>[5x]MNESVKEIPDVLKSQCGFNCLTDISHSSFNEFRQQVSEHLSWSETHDLYHDAQQAQKDNRLYEARILKRANPQLQNAVHLAILAPNAELIGYNNQFSGRASQYVAPGTVSSMFSPAAYLTELYREARNLHASDSVYYLDTRRPDLKSMALSQQNMDIELSTLSLSNELLLESIKTESKLENYTKVMEMLSTFRPSGATPYHDAYENVREVIQLQDPGLEQLNASPAIAGLMHQASLLGINASISPELFNILTEEITEGNAEELYKKNFGNIEPASLAMPEYLKRYYNLSDEELSQFIGKASNFGQQEYSNNQLITPVVNSSDGTVKVYRITREYTTNAYQMDVELFPFGGENYRLDYKFKNFYNASYLSIKLNDKRELVRTEGAPQVNIEYSANITLNTADISQPFEIGLTRVLPSGSWAYAAAKFTVEEYNQYSFLLKLNKAIRLSRATELSPTILEGIVRSVNLQLDINTDVLGKVFLTKYYMQRYAIHAETALILCNAPISQRSYDNQPSQFDRLFNTPLLNGQYFSTGDEEIDLNSGSTGDWRKTILKRAFNIDDVSLFRLLKITDHDNKDGKIKNNLKNLSNLYIGKLLADIHQLTIDELDLLLIAVGEGKTNLSAISDKQLATLIRKLNTITSWLHTQKWSVFQLFIMTSTSYNKTLTPEIKNLLDTVYHGLQGFDKDKADLLHVMAPYIAATLQLSSENVAHSVLLWADKLQPGDGAMTAEKFWDWLNTKYTPGSSEAVETQEHIVQYCQALAQLEMVYHSTGINENAFRLFVTKPEMFGAATGAAPAHDALSLIMLTRFADWVNALGEKASSVLAAFEANSLTAEQLADAMNLDANLLLQASIQAQNHQHLPPVTPENAFSCWTSINTILQWVNVAQQLNVAPQGVSALVGLDYIESMKETPTYAQWENAAGVLTAGLNSQQANTLHAFLDESRSAALSTYYIRQVAKAAAAIKSRDDLYQYLLIDNQVSAAIKTTRIAEAIASIQLYVNRALENVEENANSGVISRQFFIDWDKYNKRYSTWAGVSQLVYYPENYIDPTMRIGQTKMMDALLQSVSQSQLNADTVEDAFMSYLTSFEQVANLKVISAYHDNINNDQGLTYFIGLSETDAGEYYWRSVDHSKFNDGKFAANAWSEWHKIDCPINPYKSTIRPVIYKSRLYLLWLEQKEITKQTGNSKDGYQTETDYRYELKLAHIRYDGTWNTPITFDVNKKISELKLEKNRAPGLYCAGYQGEDTLLVMFYNQQDTLDSYKNASMQGLYIFADMASKDMTPEQSNVYRDNSYQQFDTNNVRRVNNRYAEDYEIPSSVSSRKDYGWGDYYLSMVYNGDIPTINYKAASSDLKIYISPKLRIIHNGYEGQKRNQCNLMNKYGKLGDKFIVYTSLGVNPNNSSNKLMFYPVYQYSGNTSGLNQGRLLFHRDTTYPSKVEAWIPGAKRSLTNQNAAIGDDYATDSLNKPDDLKQYIFMTDSKGTATDVSGPVEINTAISPAKVQIIVKAGGKEQTFTADKDVSIQPSPSFDEMNYQFNALEIDGSGLNFINNSASIDVTFTAFAEDGRKLGYESFSIPVTLKVSTDNALTLHHNENGAQYMQWQSYRTRLNTLFARQLVARATTGIDTILSMETQNIQEPQLGKGFYATFVIPPYNLSTHGDERWFKLYIKHVVDNNSHIIYSGQLTDTNINITLFIPLDDVPLNQDYHAKVYMTFKKSPSDG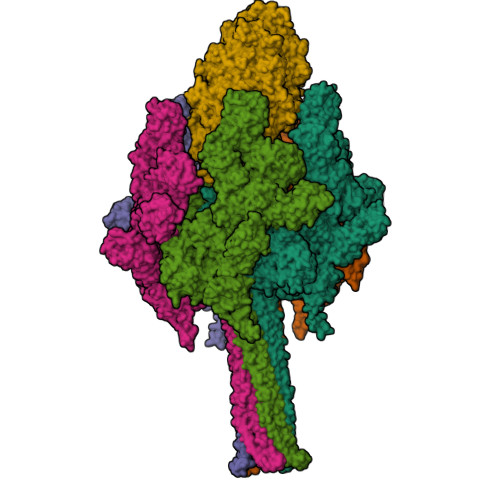TWWGPHFVRDDKGIVTINPKSILTHFESVNVLNNISSEPMDFSGANSLYFWELFYYTPMLVAQRLLHEQNFDEANRWLKYVWSPSGYIVHGQIQNYQWNVRPLLEDTSWNSDPLDSVDPDAVAQHDPMHYKVSTFMRTLDLLIARGDHAYRQLERDTLNEAKMWYMQALHLLGDKPYLPLSTTWSDPRLDRAADITTQNAHDSAIVALRQNIPTPAPLSLRSANTLTDLFLPQINEVMMNYWQTLAQRVYNLRHNLSIDGQPLYLPIYATPADPKALLSAAVATSQGGGKLPESFMSLWRFPHMLENARGMVSQLTQFGSTLQNIIERQDAEALNALLQNQAAELILTNLSIQDKTIEELDAEKTVLEKSKAGAQSRFDSYGKLYDENINAGENQAMTLRASAAGLTTAVQASRLAGAAADLVPNIFGFAGGGSRWGAIAEATGYVMEFSANVMNTEADKISQSETYRRRRQEWEIQRNNAEAELKQIDAQLKSLAVRREAAVLQKTSLKTQQEQTQSQLAFLQRKFSNQALYNWLRGRLAAIYFQFYDLAVARCLMAEQAYRWELNDDSARFIKPGAWQGTYAGLLAGETLMLSLAQMEDAHLKRDKRALEVERTVSLAEVYAGLPKDNGPFSLAQEIDKLVSQGSGSAGSGNNNLAFGAGTDTKTSLQASVSFADLKIREDYPASLGKIRRIKQISVTLPALLGPYQDVQAILSYGDKAGLANGCEALAVSHGMNDSGQFQLDFNDGKFLPFEGIAIDQGTLTLSFPNASMPEKGKQATMLKTLNDIILHIRYTIK;> MQNSQDFSITELSLPKGGGAITGMGEALTPTGPDGMAALSLPLPISAGRGYAPAFTLNYNSGAGNSPFGLGWDCNVMTIRRRTHFGVPHYDETDTFLGPEGEVLVVADQPRDESTLQGINLGATFTVTGYRSRLESHFSRLEYWQPKTTGKTDFWLIYSPDGQVHLLGKSPQARISNPSQTTQTAQWLLEASVSSRGEQIYYQYRAEDDTGCEADEITHHLQATAQRYLHIVYYGNRTASETLPGLDGSAPSQADWLFYLVFDYGERSNNLKTPPAFSTTGSWLCRQDRFSRYEYGFEIRTRRLCRQVLMYHHLQALDSKITEHNGPTLVSRLILNYDESAIASTLVFVRRVGHEQDGNVVTLPPLELAYQDFSPRHHAHWQPMDVLANFNAIQRWQLVDLKGEGLPGLLYQDKGAWWYRSAQRLGEIGSDAVTWEKMQPLSVIPSLQSNASLVDINGDGQLDWVITGPGLRGYHSQRPDGSWTRFTPLNALPVEYTHPRAQLADLMGAGLSDLVLIGPKSVRLYANTRDGFAKGKDVVQSGEITLPVPGADPRKLVAFSDVLGSGQAHLVEVSATKVTCWPNLGRGRFGQPITLPGFSQPATEFNPAQVYLADLDGSGPTDLIYVHTNRLDIFLNKSGNGFAEPVTLRFPEGLRFDHTCQLQMADVQGLGVASLILSVPHMSPHHWRCDLTNMKPWLLNEMNNNMGVHHTLRYRSSSQFWLDEKAAALTTGQTPVCYLPFPIHTLWQTETEDEISGNKLVTTLRYARGAWDGREREFRGFGYVEQTDSHQLAQGNAPERTPPALTKNWYATGLPVIDNALSTEYWRDDQAFAGFSPRFTTWQDNKDVPLTPEDDNSRYWFNRALKGQLLRSELYGLDDSTNKHVPYTVTEFRSQVRRLQHTDSRYPVLWSSVVESRNYHYERIASDPQCSQNITLSSDRFGQPLKQLSVQYPRRQQPAINLYPDTLPDKLLANSYDDQQRQLRLTYQQSSWHHLTNNTVRVLGLPDSTRSDIFTYGAENVPAGGLNLELLSDKNSLIADDKPREYLGQQKTAYTDGQNTTPLQTPTRQALIAFTETTVFNQSTLSAFNGSIPSDKLSTTLEQAGYQQTNYLFPRTGEDKVWVAHHGYTDYGTAAQFWRPQKQSNTQLTGKITLIWDANYCVVVQTRDAAGLTTSAKYDWRFLTPVQLTDINDNQHLITLDALGRPITLRFWGTENGKMTGYSSPEKASFSPPSDVNAAIELKKPLPVAQCQVYAPESWMPVLSQKTFNRLAEQDWQKLYNARIITEDGRICTLAYRRWVQSQKAIPQLISLLNNGPRLPPHSLTLTTDRYDHDPEQQIRQQVVFSDGFGRLLQAAARHEAGMARQRNEDGSLIINVQHTENRWAVTGRTEYDNKGQPIRTYQPYFLNDWRYVSNDSARQEKEAYADTHVYDPIGREIKVITAKGWFRRTLFTPWFTVNEDENDTAAEVKKVKMPGSRPMKNIDPKLYQKTPTVSVYDNRGLIIRNIDFHRTTANGDPDTRITRHQYDIHGHLNQSIDPRLYEAKQTNNTIKPNFLWQYDLTGNPLCTESIDAGRTVTLNDIEGRPLLTVTATGVIQTRQYETSSLPGRLLSVAEQTPEEKTSRITERLIWAGNTEAEKDHNLAGQCVRHYDTAGVTRLESLSLTGTVLSQSSQLLIDTQEANWTGDNETVWQNMLADDIYTTLSTFDATGALLTQTDAKGNIQRLAYDVAGQLNGSWLTLKGQTEQVIIKSLTYSAAGQKLREEHGNDVITEYSYEPETQRLIGIKTRRPSDTKVLQDLRYEYDPVGNVISIRNDAEATRFWHNQKVMPENTYTYDSLYQLISATGREMANIGQQSHQFPSPALPSDNNTYTNYTRTYTYDRGGNLTKIQHSSPATQNNYTTNITVSNRSNRAVLSTLTEDPAQVDALFDAGGHQNTLISGQNLNWNTRGELQQVTLVKRDKGANDDREWYRYSGDGRRMLKINEQQASNNAQTQRVTYLPNLELRLTQNSTATTEDLQVITVGEAGRAQVRVLHWESGKPEDIDNNQLRYSYDNLIGSSQLELDSEGQIISEEEYYPYGGTALWAARNQTEASYKTIRYSGKERDATGLYYYGYRYYQPWIGRWLSSDPAGTIDGLNLYRMVRNNPVTLLDPDGLMPTIAERIAALKKNKVTDSAPSPANATNVAINIRPPVAPKPSLPKASTSSQPTTHPIGAANIKPTTSGSSIVAPLSPVGNKSTSEISLPESAQSSSSSTTSTNLQKKSFTLYRADNRSFEEMQSKFPEGFKAWTPLDTKMARQFASIFIGQKDTSNLPKETVKNISTWGAKPKLKDLSNYIKYTKDKSTVWVSTAINTEAGGQSSGAPLHKIDMDLYEFAIDGQKLNPLPEGRTKNMVPSLLLDTPQIETSSIIALNHGPVNDAEISFLTTIPLKNVKPHKR>AAAA[14x];>[14x]MMGYIPYVIENTDRGERSYDIYSRLLKDRIVLLSGEINDSVASSIVAQLLFLEAEDPEKDIGLYINSPGGVITSGLSIYDTMN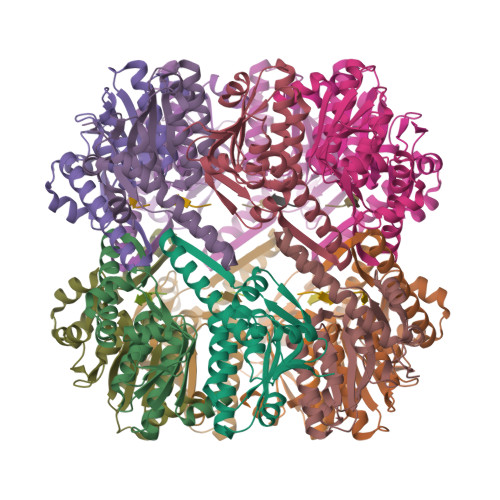FIRPDVSTICIGQAAAMGAFLLSCGAKGKRFSLPHSRIMIHQPLGGAQGQASDIEIISNEILRLKGLMNSILAQNSGQSLEQIAKDTDRDFYMSAKEAKEYGLIDKVLQKNVK>[2x]MNNNDIEYNAPSEIKYIDVVNTYDLEEEASK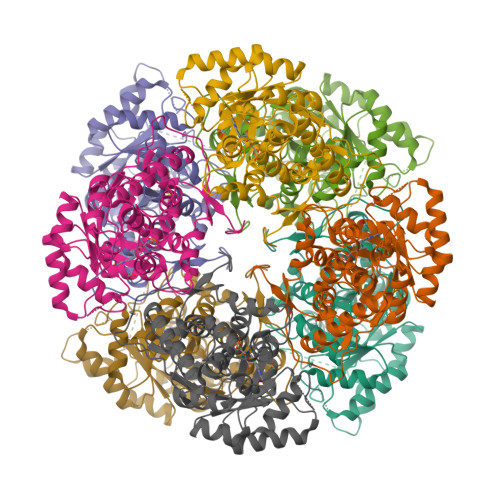VVPHGGFNYIAGASGDEWTKRANDRAWKHKLLYPRLAQDVEAPDTSTEILGHKIKAPFIMAPIAAHGLAHTTKEAGTARAVSEFGTIMSISAYSGATFEEISEGLNGGPRWFQIYMAKDDQQNRDILDEAKSDGATAIILTADSTVSGNRDRDVKNKFVYPFGMPIVQRYLRGTAEGMSLNNIYGASKQKISPRDIEEIAGHSGLPVFVKGIQHPEDADMAIKRGASGIWVSNHGARQLYEAPGSFDTLPAIAERVNKRVPIVFDSGVRRGEHVAKALASGADVVALGRPVLFGLALGGWQGAYSVLDYFQKDLTRVMQLTGSQNVEDLKGLDLFDNPYGYEY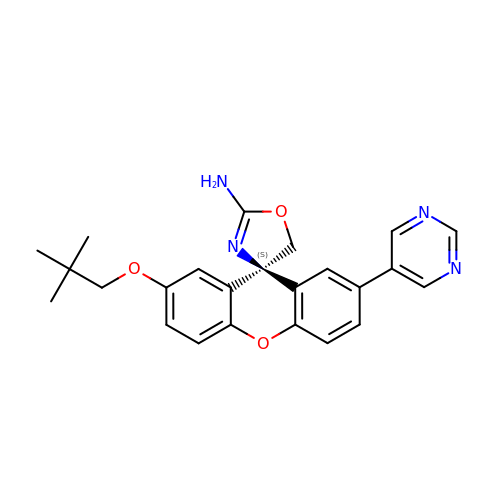(4S)-2'-(2,2-dimethylpropoxy)-7'-(pyrimidin-5-yl)spiro[1,3-oxazole-4,9'-xanthen]-2-amine | C24 H24 N4 O3 | CHZHWZAKWGFQNL-DEOSSOPVSA-N>[2x]GSHMIKSSFKAQPFLVRNTILCPNDKRSFTEYTQVIETVSKNKVFLEQLLLANPKLYDVMQKYNAGLLKKKRVKKLFESIYKYYKRSYLRSTPFGLFSETSIGVFSKSSQYKLMGKTTKGIRLDTQWLIRLVHKMEVDFSKKLSFTRNNANYKFGDRVFQVYTINSSELEECNIKYTNVYQIISEFCENDYQKYEDICETVTLCYGDEYRELSEQYLGSLIVNHYLISNLQKDLLSDFSWNTFLTKVEAIDEDKKYIIPLKKVQKFIQEYSEIEIGEGIEKLKEIYQEMSQILENDNYIQIDLISDSEINFDVKQKQQLEHLAEFLGNTTKSVRRTYLDDYKDKFIEKYGVDQEVQITELFDSTFGIGAPYNYNHPRNDFYESEPSTLYYSEEEREKYLSMYVEAVKNHNVINLDDLESHYQKMDLEKKSELQGLELFLNLAKEYEKDIFILGDIVGNNNLGGASGRFSALSPELTSYHRTIVDSVERENENKEITSCEIVFLPENIRHANVMHTSIMRRKVLPFFTSTSHNEVLLTNIYIGIDEKEKFYARDISTQEVLKFYITSMYNKTLFSNELRFLYEISLDDKFGNLPWELIYRDFDYIPRLVFDEIVISPAKWKIWGRDVNSKMTIRELIQSKEIPKEFYIVNGDNKVYLSQKNPLDMEILESAIKKSSKRKDFIELQEYFEDENIINKGEKGRVADVVVPFIRTRALGNEGRAFIREKRVSVERREKLPFNEWLYLKLYISINRQNEFLLSYLPDIQKIVANLGGNLFFLRYTDPKPHIRLRIKCSDLFLAYGSILEILKRSRKNRIMSTFDISIYDQEVERYGGFDTLELSEAIFCADSKIIPNLLTLIKDTNNDWKVDDVSILVNYLYLKCFFQNDNKKILNFLNLVSTKKVKENVNEKIEHYLKLLKVNNLGDQIFYDKNFKELKHAIKNLFL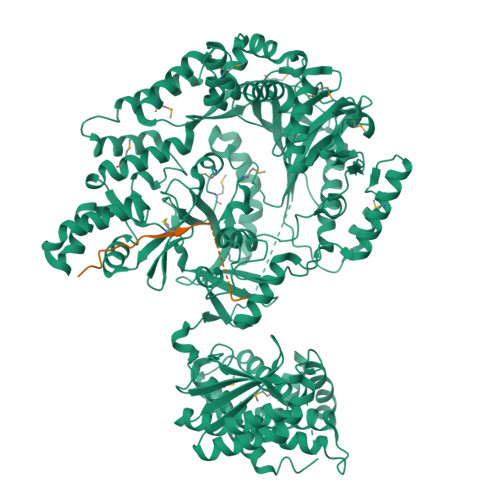KMIAQDFELQKVYSIIDSIIHVHNNRLIGIERDKEKLIYYTLQRLFVSEEYMK;>STKDFNLDLVCVSKKDSGASPRITXISLATPGAK[2x]> MSDSLLVRTSRDGDQFHYLWAARRALRLLEPQSTLVALTIEGASTTEMGSQPVVEDGEELIDIAEYYGSNELATATTVRYMQLKHSTMHSDTPFPPSGLQKTIEGFATRYKALIQKIPVETLRTKLEFWFVTNRPVSSSFSEAINDAANQHVTRHPHDLAKLEKFTGLQGAELSIFCQLLHIEGQQDDLWSQRNILLRESAGYLPDLDTEAPLKLKELVNRKALTESAANPSITRMDVLRALGVDETDLFPAPCRIERIENSVSRTQEATLVQRVVEAFGAPVIIHADAGVGKSIFSTHIEEHLPTGSVSILYDCFGLGQYRNASSYRHHHRTALVQMANEMASRGLCHPLIPNAGTGISQ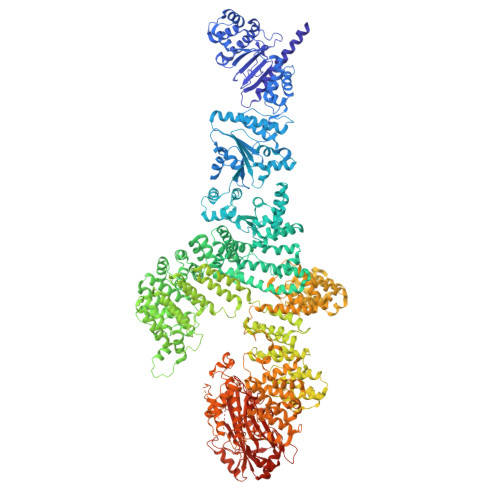YMRAFLHRLSQSISILRASEPLAVLCIIIDAADNAQMAAEEIGETRSFIKDLIREKLPDGVCLVALCRPYRRELLDPPPEALTLSLQTFNRDETAAHLHQKFPDASESDVDEFHRLSSCNPRVQALSLSQNLPLNDTLRLLGPNPKTVEDTIGEVLEKSIARLRDTAGISERAQIDTICSALAILRPLIPLSVLSAISGVAGSAIKSFALDLGRPLIVSGETIQFFDEPAETWFQRRFRPSAADLHQFITKLRPLTKDSSYAASVLPALMLEGNQLSELIELAISSQALPETSAVERRDIELQRLQFALKAALRTGRYQDAAKLALKAGGECAGDNRQRVLLRDNIDLAAKFVGSNGVQELVSRNAFPDTGWPGSRNAYYAAILSEYPELSGEARSRLRLTMEWLTNWSQLPDDERSRQNVTDQDRAVMLIACLNIHGAEAAARELRRWRPRKLSFDAGKIVAMQLLAHARYDELDQLAIAAGNDISLVMGIVLEARKLHRPVAEQAIRRTWRLLKSQRVSIKDRNHANNQTIAAITGMVEMALIQSVCTESESIQLLDRYLPKVPPYALTSEYSKERVAYVRAYALQANLMGSQLALSDLASTEVKKELMAEKRHGESDDLRQLKQYSGVLIPWYNLWAKVILGKTRKADLESELSDTQKESTAIKGHSYSEHSLSSNEIANVWFDILIEAGNVSKDDVENIIKWSQHKGNRVFTPTLHRFSSVCAEISGLGELSYHFAELALSLWRDEHSDAQIKADGYIDLSRSLISLDEPEAKEYFNQAIEVTNKLGDENLSRWEAILDLAEYVAGKTQVPPEISYKLARCAELTREYVDRDKHFAWSDTVEILAELCPSSALAIISRWRDRTFGNHRSILAWTIEHLVKKNKINALDALPLITFENDWHKCDLLDSVLSSCTDDKDKIMAFEVVYHYTKFNVQNIQNLKKLDAISTSLGIEHTELKERISGLQHTETVSKKSSLSSNDNEQGHDQEWESIFKDCDLSSIDGISAAYEKFRNVPEFYSKETFIKKAISRVKTGKECSFITAIGAIFHWGLYDFKYILESIPDEWTSRLSIKTTLAGLIKEYCQRFCMRIRKSRVYEIFPFSLASRLSGISEKEIFGITLEAIAESPEPANSDRLFSLPGLLVSKLESNEALDVLSYALDLFDEVLKDEDGDGPWNEKLSPPTHVEDSLAGYIWARLGSPEAEMRWQAAHAVLALCRMSRTCVIQGIFQHAINATTLPFCDRNLPFYTLHAQLWLMIAAARVALDDGKSLIPNIGYFYHYATTDQPHVLIRHFAARTLLALHDSDLISIPAQEENKLRNINQSTTLPVLDKVEDHRGEDSYTFGIDFGPYWLKPLGRCFGVSQKQLEPEMLRIIRDVLGFKGSRNWDEDERNKRRYYQDRDNHHSHGSYPRVDDYHFYLSYHAMFMTAGQLLATKPLVGSDYDDVEDVFQDWLRRHDISRNDHRWLADRRDIPPKERSSWLNSSSDNRDEWLASISENVFNETLCPSPGLLTLWGRWSDVCSDRKESIIVHSALVSPERSLSLLRALQTTKNVYDYKIPDAGDNLEIDHAHYQLKGWIKDIAEYCGIDEFDPWAGNVRFPIPEPASFIIDAMKLTTDKDHRVWYSPSDVEPAMISSIWGHLSGKNDEEKSHGYRLCASIHFIKSALETFNMDLILEVDVDRYSRNSRYERNNENELDNIPSSTRLFLFRHDGTIHTLYGNYRNGEKTS>[2x]IVGGTASVRGEWPWQVTLHTTSPTQRHLCGGSIIGNQWILTAAHCFYGVESPKI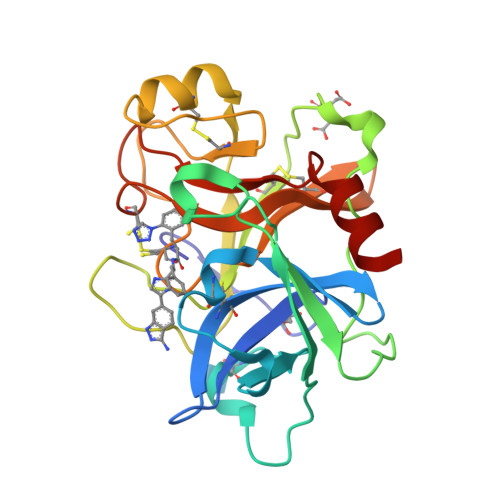LRVYSGILNQSEIKEDTSFFGVQEIIIHDQYKMAESGYDIALLKLETTVNYTDSQRPISLPSKGDRNVIYTDCWVTGWGYRKLRDKIQNTLQKAKIPLVTNEECQKRYRGHKITHKMICAGYREGGKDACKGDSGGPLSCKHNEVWHLVGITSWGEGCAQRERPGVYTNVVEYVDWILEKTQAV>MLGEREKLLRLEEELHKRVVGQDEAIRAVADAIRRARAGLKDPNRPIGSFLFLGPTGVGKTELAKTLAATLFDTEEAMIRIDMTEYMEKHAVSRLIGAPPGYVGYEEGGQLTEAVRRRPYSVILFDAIEKAHPDVFNILLQMLDDGRLTDSHGRTVDFRNTVIIMTSNLGSPLILEGLQKGWPYERIRDEVFKVLQQHFRPEFLNRLDEIVVFRPLTKEQIRQIVEIQMSYLRARLAEKRISLELTEAAKDFLAERGYDPVFGARPLRRVIQRELE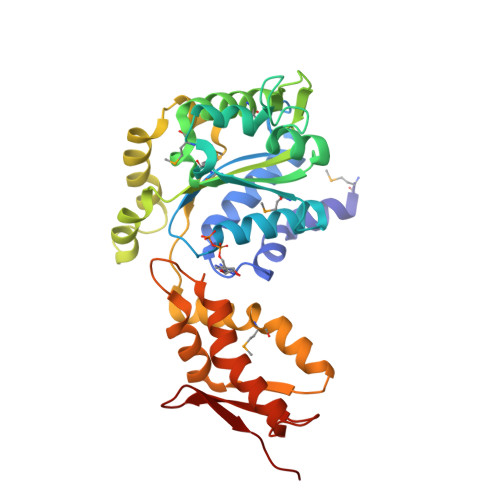TPLAQKILAGEVKEGDRVQVDVGPAGLVFAVPARV[3x]>[7x]MSDLDRLASRAAIQDLYSDQLIGVDKRQEGRLASIWWDDAEWTIEGIGTYKGPEGALDLANNVLWPMYHETIHYGTNLRLEFVSADKVNGIGDVLCLGNLVEGNQSILIAAVYTNEYERRDGVWKFSKLNGCMNYFTPLAGIHFAPPGIHFAPSGA

LinA variants exhibit considerable differences in their thermostability and enantioselectivity. The active site of LinA is largely hydrophobic in character and is located in the characteristic cavity of the tertiary barrel fold. Among other things, H73 functions as a base that abstracts the proton of γ-HCH, leading to its dehydrochlorination. The C-terminal segment has been implicated in the catalytic mechanism of LinA proteins, where based on its spatial position, the enzyme is thought to be in an ‘open’ or ‘closed’ form.

Here we show that LinA-type2 exhibits preference for (+) enantiomer of α-HCH and also report its crystal structure. Crystals of LinA-type2 that diffracted to a moderate resolution of 3.5 Å in the space group P6322 were obtained. Molecular replacement studies revealed that the crystal has seven subunits in the asymmetric unit. The structure of the -type2 protein is understandably highly conserved compared to the -type1 protein and therefore it was unanticipated that it would exhibit different enantiomer specificity for α-HCH compared to the -type1 protein. Analysis of the active site residues itself shows that the -type2 protein exhibits several differences including K20Q, F68Y, C71T, L96C F113Y, R129L and A131G, compared to -type1 protein. The main differences T133M, F68Y and A131G, present vicinal to the entrance to the active site in -type2 protein might lead to overall reduced substrate accessibility. Further analysis of the active site and interactions of the substrates in the respective docked complexes were carried out. It was identified that residue changes K20Q, F68Y, C71T, L96C, F113Y, A131G and T133M in -type2 are vicinal to the docked HCH moiety and could conceivably alter the contours of the active site to enforce enantioselectivity. Thermostability of LinAs, as measured by loss of activity after incubation at 60°C for different time periods, revealed that while >50% activity of LinA-type1 was lost after one hour, activity of LinA-type2 continued to remain unchanged even after two hours also [6]. Amongst the ten residues that differ between -type1 and -type2 proteins, two residues viz. Q20 and G23 are important determinants for this property as seen by measurement of enzyme activity and CD-spectroscopy experiments at varying temperatures of a series of LinA-type2 mutants.> GGDGRKKRKRCGTCEPCRRLENCGACTSCTNRRTHQICKLR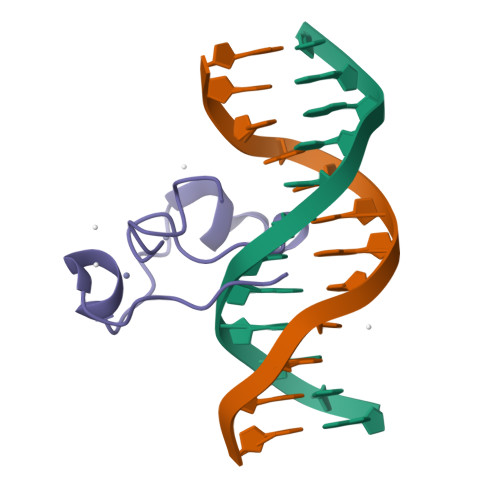KCEVLKKKVGL1,2-DILAUROYL-SN-GLYCERO-3-PHOSPHATE | C27 H52 O8 P | 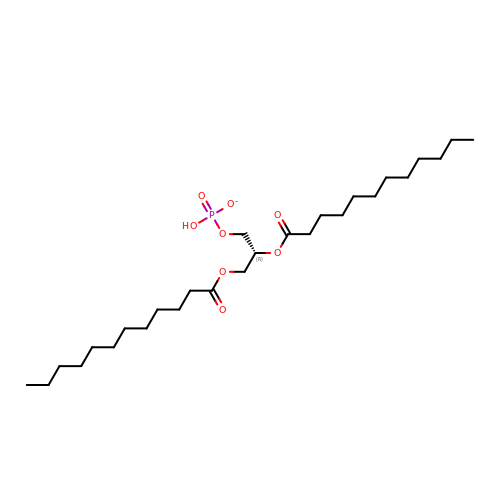OKLASJZQBDJAPH-RUZDIDTESA-M>[4x]SASASAMLSRKGIIPEEYVLTRLAEDPAEPRYRARQRRARFVSKKGNCNVAHKNIREQGRFLQDVFTTLVDLKWPHTLLIFTMSFLCSWLLFAMAWWLIAFAHGDLAPSEGTAEPCVTSIHSFSSAFLFSIEVQVTIGFGGRMVTEECPLAILILIVQNIVGLMINAIMLGCIFMKTAQAHRRAETLIFSKHAVIALRHGRLCFMLRVGDLRKSMIISATIHMQVVRKTTSPEGEVVPLHQVDIPMENGVGGNSIFLVAPLIIYHVIDANSPLYDLAPSDLHHHQDLEIIVILEGVVETTGITTQARTSYLADEILWGQRFVPIVAEEDGRYSVDYSKFGNTIKVPTPLCTARQLDEDHSLLEALTLASARGPLRKRSVPMAKAKPKFSISPDSLSSNSLEVLFQG;>[4x]MPLAFCGSENHSAAYRVDQGVLNNGCFVDALNVVPHVFLLFITFPILFIGWGSQSSKVHIHHSTWLHFPGHNLRWILTFMLLFVLVCEIAEGILSDGVTESHHLHLYMPAGMAFMAAVTSVVYYHNIETSNFPKLLIALLVYWTLAFITKTIKFVKFLDHAIGFSQLRFCLTGLLVILYGMLLLVEVNVIRVRRYIFFKTPREVKPPEDLQDLGVRFLQPFVNLLSKGTYWWMNAFIKTAHKKPIDLRAIGKLPIAMRALTNYQRLCEAFDAQVRKDIQGTQGARAIWQALSHAFGRRLVLSSTFRILADLLGFAGPLCIFGIVDHLGKENDVFQPKTQFLGVYFVSSQEFLANAYVLAVLLFLALLLQRTFLQASYYVAIETGINLRGAIQTKIYNKIMHLSTSNLSMGEMTAGQICNLVAIDTNQLMWFFFLCPNLWAMPVQIIVGVILLYYILGVSALIGAAVIIL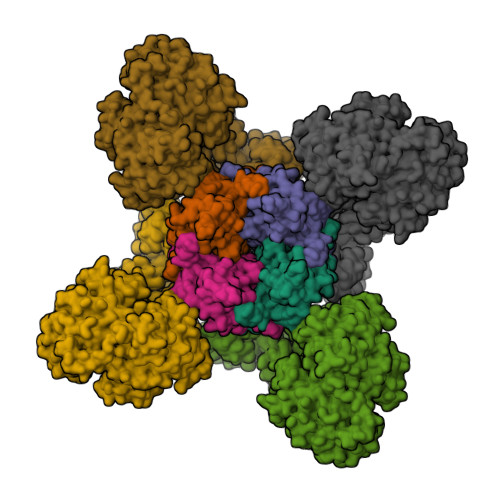LAPVQYFVATKLSQAQRSTLEYSNERLKQTNEMLRGIKLLKLYAWENIFRTRVETTRRKEMTSLRAFAIYTSISIFMNTAIPIAAVLITFVGHVSFFKEADFSPSVAFASLSLFHILVTPLFLLSSVVRSTVKALVSVQKLSEFLSSAEIREEQCAPHEPTPQGPASKYQAVPLRVVNRKRPAREDCRGLTGPLQSLVPSADGDADNCCVQIMGGYFTWTPDGIPTLSNITIRIPRGQLTMIVGQVGCGKSSLLLAALGEMQKVSGAVFWSSLPDSEIGEDPSPERETATDLDIRKRGPVAYASQKPWLLNATVEENIIFESPFNKQRYKMVIEACSLQPDIDILPHGDQTQIGERGINLSGGQRQRISVARALYQHANVVFLDDPFSALDIHLSDHLMQAGILELLRDDKRTVVLVTHKLQYLPHADWIIAMKDGTIQREGTLKDFQRSECQLFEHWKTLMNRQDQELEKETVTERKATEPPQGLSRAMSSRDGLLQDEEEEEEEAAESEEDDNLSSMLHQRAEIPWRACAKYLSSAGILLLSLLVFSQLLKHMVLVAIDYWLAKWTDSALTLTPAARNCSLSQECTLDQTVYAMVFTVLCSLGIVLCLVTSVTVEWTGLKVAKRLHRSLLNRIILAPMRFFETTPLGSILNRFSSDCNTIDQHIPSTLECLSRSTLLCVSALAVISYVTPVFLVALLPLAIVCYFIQKYFRVASRDLQQLDDTTQLPLLSHFAETVEGLTTIRAFRYEARFQQKLLEYTDSNNIASLFLTAANRWLEVRMEYIGACVVLIAAVTSISNSLHRELSAGLVGLGLTYALMVSNYLNWMVRNLADMELQLGAVKRIHGLLKTEAESYEGLLAPSLIPKNWPDQGKIQIQNLSVRYDSSLKPVLKHVNALIAPGQKIGICGRTGSGKSSFSLAFFRMVDTFEGHIIIDGIDIAKLPLHTLRSRLSIILQDPVLFSGTIRFNLDPERKCSDSTLWEALEIAQLKLVVKALPGGLDAIITEGGENFSQGQRQLFCLARAFVRKTSIFIMDEATASIDMATENILQKVVMTAFADRTVVTIAHRVHTILSADLVIVLKRGAILEFDKPEKLLSRKDSVFASFVRADK> MERRRLLHDGRWFTPPVLYGSARRGLKTLDVREYRPLAMPIEFRFYQRYANHPNRQSGIQFLTHYNTHQRFRVNKDYIDYMHWGKEQGQARLPHRHQRVAFDFNDQLHPTRIGTPEDGGNANHCYPEDGEDGSYAWFASQDPTFGHHPDLSSSFDPNYRVFSHPEHWNKMFTKRRPGEGDIDLSVLPSRSLLGPLMAHSDTKGIPYFKVDNRGHSNGRVPGVNAPFFGEFDQKMMQAMSRPLNANRTITGNDGRFSKTIMINEPQCNQALSAKTASELSKEIDKATNAVYSKLSVLEAAQSGLTDYFCGGLNFEIVGFELHMAAMLRERAAAILERSGAGGLPSASSATLSSSSTTRRCAMLLEKADEREVNKLLRDASRYEDRVDDALRQHASLIWRVYTAPRPLMTLTNGKCRGTGCGLSLFAKYCALKDSSEFIFDGPNVGITPYGGMTRLLARPETSLKYPGLAEFVVLTGASLFAGDALRLGWTDLFTTIPDMTYHIKEWFDTTEHMHNDAVAWQLGHLLETCFKMKESHSSAMERAAITPTRARWVEDAFADQPSVNDIMRTLTEIEQLPFQSTHNTSDESHITPYTLGSVAAGVQRLGEHRLRYTLSPWD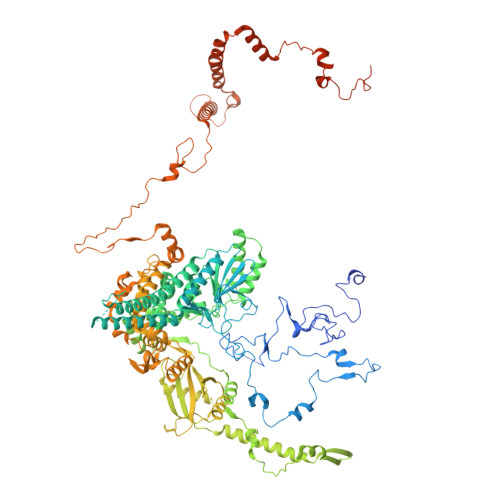ITPPEDSVVLKHTSEMFRAYVLERRGATDVVTHRDAERAAAWSQQRQREYDAYCSLKEAPHPRHVYARLEGCEGKIVSFEFVFEISCRRSGPQGTDEVLQATTISRLKSRILDALGMPRDRNIDLGWYLPTLDTCPIHSDEELMQVLHTDPGIEDPKEKLRYPPIYFIVKRCTLYFSEWAYAVKHQLLLQSPFALRAAFGLLQEVRGDGAAENVMPLAETLGTEFKYFTRLMRRPDFYRVGVHTDKSVEKWEEIKEERRHNIHHTHRPTRPLPDFEEVFERDVEIDGHRFVLRPRWNPRTLQDVDDSDILRLRAPLTYDMDSTAALHVPTHCGKASRLAGMLQDAGGVQVLDGLGEVDDKGEPKVPPLQSNASVPTNVSFYEMARHPWEDRASSWRRDGFTEGSLEYFESQYRSAERAVYDEEGRGVRNYWPSRDAVEGIAQEEENDAQLLQERLFNTLETAGTSVEPWARNLRLNATTGKFGYKTEIATQEEKIYDDEYYRWFIQPGRHPNPSGLTLNGRKGQFEEGHSRDEELERMWRKVVADGNNDFAATTSGMPVYDEDAKNAEDSYAAGDDVDVVTTDANVPVDGDDSS> MAAQVTLEDALSNVDLLEELPLPDQQPCIEPPPSSLLYQPNFNTNFEDRNAFVTGIARYIEQATVHSSMNEMLEEGQEYAVMLYTWRSCSRAIPQVKCNEQPNRVEIYEKTVEVLEPEVTKLMNFMYFQRNAIERFCGEVRRLCHAERRKDFVSEAYLITLGKFINMFAVLDELKNMKCSVKNDHSAYKRAAQFLRKMADPQSIQESQNLSMFLANHNKITQSLQQQLEVISGYEELLADIVNLCVDYYENRMYLTPSEKHMLLKVMGFGLYLMDGSVSNIYKLDAKKRINLSKIDKYFKQLQVVPLFGDMQIELARYIKTSAHYEENKSRWTCTSSGSSPQYNICEQMIQIREDHMRFISELARYSNSEVVTGSGRQEAQKTDAEYRKLFDLALQGLQLLSQWSAHVMEVYSWKLVHPTDKYSNKDCPDSAEEYERATRYNYTSEEKFALVEVIAMIKGLQVLMGRMESVFNHAIRHTVYAALQDFSQVTLREPLRQAIKKKKNVIQSVLQAIRKTVCDWETGHEPFNDPALRGEKDPKSGFDIKVPRRAVGPSSTQLYMVRTMLESLIADKSGSKKTLRSSLEGPTILDIEKFHRESFFYTHLINFSETLQQCCDLSQLWFREFFLELTMGRRIQFPIEMSMPWILTDHILETKEASMMEYVLYSLDLYNDSAHYALTRFNKQFLYDEIEAEVNLCFDQFVYKLADQIFAYYKVMAGSLLLDKRLRSECKNQGATIHLPPSNRYETLLKQRHVQLLGRSIDLNRLITQRVSAAMYKSLELAIGRFESEDLTSIVELDGLLEINRMTHKLLSRYLTLDGFDAMFREANHNVSAPYGRITLHVFWELNYDFLPNYCYNGSTNRFVRTVLPFSQEFQRDKQPNAQPQYLHGSKALNLAYSSIYGSYRNFVGPPHFQVICRLLGYQGIAVVMEELLKVVKSLLQGTILQYVKTLMEVMPKICRLPRHEYGSPGILEFFHHQLKDIVEYAELKTVCFQNLREVGNAILFCLLIEQSLSLEEVCDLLHAAPFQNILPRVHVKEGERLDAKMKRLESKYAPLHLVPLIERLGTPQQIAIAREGDLLTKERLCCGLSMFEVILTRIRSFLDDPIWRGPLPSNGVMHVDECVEFHRLWSAMQFVYCIPVGTHEFTVEQCFGDGLHWAGCMIIVLLGQQRRFAVLDFCYHLLKVQKHDGKDEIIKNVPLKKMVERIRKFQILNDEIITILDKYLKSGDGEGTPVEHVRCFQPPIHQSLASS;> MSRSVLQPSQQKLAEKLTILNDRGVGMLTRLYNIKKACGDPKAKPSYLIDKNLESAVKFIVRKFPAVETRNNNQQLAQLQKEKSEILKNLALYYFTFVDVMEFKDHVCELLNTIDVCQVFFDITVNFDLTKNYLDLIITYTTLMILLSRIEERKAIIGLYNYAHEMTHGASDREYPRLGQMIVDYENPLKKMMEEFVPHSKSLSDALISLQMVYPRRNLSADQWRNAQLLSLISAPSTMLNPAQSDTMPCEYLSLDAMEKWIIFGFILCHGILNTDATALNLWKLALQSSSCLSLFRDEVFHIHKAAEDLFVNIRGYNKRINDIRECKEAAVSHAGSMHRERRKFLRSALKELATVLSDQPGLLGPKALFVFMALSFARDEIIWLLRHADNMPKKSADDFIDKHIAELIFYMEELRAHVRKYGPVMQRYYVQYLSGFDAVVLNELVQNLSVCPEDESIIMSSFVNTMTSLSVKQVEDGEVFDFRGMRLDWFRLQAYTSVSKASLGLADHRELGKMMNTIIFHTKMVDSLVEMLVETSDLSIFCFYSRAFEKMFQQCLELPSQSRYSIAFPLLCTHFMSCTHELCPEERHHIGDRSLSLCNMFLDEMAKQARNLITDICTEQCTLSDQLLPKHCAKTISQAVNKKSKKQTGKKGEPEREKPGVESMRKNRLVVTNLDKLHTALSELCFSINYVPNMVVWEHTFTPREYLTSHLEIRFTKSIVGMTMYNQATQEIAKPSELLTSVRAYMTVLQSIENYVQIDITRVFNNVLLQQTQHLDSHGEPTITSLYTNWYLETLLRQVSNGHIAYFPAMKAFVNLPTENELTFNAEEYSDISEMRSLSELLGPYGMKFLSESLMWHISSQVAELKKLVVENVDVLTQMRTSFDKPDQMAALFKRLSSVDSVLKRMTIIGVILSFRSLAQEALRDVLSYHIPFLVSSIEDFKDHIPRETDMKVAMNVYELSSAAGLPCEIDPALVVALSSQKSENISPEEEYKIACLLMVFVAVSLPTLASNVMSQYSPAIEGHCNNIHCLAKAINQIAAALFTIHKGSIEDRLKEFLALASSSLLKIGQETDKTTTRNRESVYLLLDMIVQESPFLTMDLLESCFPYVLLRNAYHAVYKQSVTSSA;> MPLVKRNIDPRHLCHTALPRGIKNELECVTNISLANIIRQLSSLSKYAEDIFGELFNEAHSFSFRVNSLQERVDRLSVSVTQLDPKEEELSLQDITMRKAFRSSTIQDQQLFDRKTLPIPLQETYDVCEQPPPLNILTPYRDDGKEGLKFYTNPSYFFDLWKEKMLQDTEDKRKEKRKQKQKNLDRPHEPEKVPRAPHDRRREWQKLAQGPELAEDDANLLHKHIEVANGGGSGGSGGSGGSGGSGGSKRHPSTLPVISDARSVLLEAIRKGIQLRKVEEQREQEAKHERIENDVATILSRRIAVEYSDSEDDSEFDEVDWLE;> MAGQEDPVQREIHQDWANREYIEIITSSIKKIADFLNSFDMSCRSRLATLNEKLTALERRIEYIEARVTKGETLT;> MAELQMLLEEEIPGGRRALFDSYTNLERVADYCENNYIQSADKQRALEETKAYTTQSLASVAYLINTLANNVLQMLDIQASQLRRMESSINHISQTVDIHKEKVARREIGILTTNKNTSRTHKIIAPANLERPVRYIRKPIDYTILDDIGHGVKVSTQ

The Rho-family GTPase Rac1 activates the WAVE regulatory complex (WRC) to drive Arp2/3 complex-mediated actin polymerization in many essential processes. The WASP-family member WAVE exists exclusively in a 400-kDa, hetero-pentameric assembly named the WAVE Regulatory Complex (WRC). The studied complex is composed of a trimer formed by WAVE1, Abi2, and HSPC300, and a dimer formed by Sra1 and Nap1 subunits. Rac1 binds to WRC at two distinct sites—the A and D sites.

Using cryo-EM we determined structures of both WRCD-Rac1 and WRCAD-Rac1, as well as WRCapo (WRC without tethered Rac1) to ~3 Å resolutions. The overall structures of WRC in these three complexes were similar to the previous crystal structure (WRCxtal), with a root-mean-square deviation (r.m.s.d.) of 0.83–1.22 Å. 187-230, which was not included in the previous WRCxtal construct, did not show any density in the cryo-EM reconstructions, suggesting that this region is disordered in WRC. By contrast, in WRCAD-Rac1, the density for the W and C helices and part of the meander region were not observed in the reconstructed map, suggesting that upon Rac1 binding to the A site, these sequences were destabilized and released from the WRC. Consistent with these observations, the pyrene-actin polymerization assay showed both WRCapo and WRCD-Rac1 were autoinhibited and could be activated by the addition of free Rac1 (blue curves), whereas WRCAD-Rac1 was basally active (solid blue curve).> GSFVGSIDQGTTSSRFLIFNGEGNPVASHQIEFENLYPKSGWHEQDPYELLNSVQQCIDGAMHKFASLGYSKENIRAIGITNQRETTVVWDSVTGEPLHNAIVWPDTRTSALVRELKARQSADSLLELCGLPLSTYPSSVKLLWLIQNVDAVKQAYEEGRLAFGTVDSWLIYKLNGGAQAERPIHVTDSTNASRTMFMNLRTLQYDDKLLGFFGIDRNKIKLPKIVPSSDPEAFGKVATGALAGVPIAGCLGDQSSALVGQCGFSPGQAKNTYGTGCFLLYNVGTEPVISKYGLLATVAYDFGRGRKPVYALEGSIAVAGAGITFLMNNLGFAPKPSEINALAESVLDNGGVVFVTAFSGLFAPYWIDDAKGTLFGITQHTTKGHIARATLEATCYQTRAILDAMEKDSGHKLESLAVDGGLSASDLCMQTQADISGIPVDRPRMRETTALGAAIAAGLATGVWRELDHVKESIAGGANGNGKKNAREVFYPKMDRKKAERLFRKWEQAVEMSRGWVREQEEEDGE

Here, we report the first structure of glycerol kinase from the thermophilic filamentous fungus Chaetomium thermophilum (CtGK). Glycerol kinase (EC 2.7.1.30) catalyzes the transfer of phosphate moiety from ATP to glycerol to form glycerol 3-phosphate (G3P). Overall, the CtGK polypeptide chain can be divided into two distinct domains classified by Pfam as FGGY_N (residues 65–325) and FGGY_C (residues 331–583) connected by a flexible region. A similar case is found in CtGK, which forms extended dimers via the interaction between the C-terminal domains with a prominent contribution from hydrophobic residues (Phe422, Gly436, Phe389, Leu394, Thr437, Phe439, Gly440, Ile441, Thr437, Thr445, Leu438, Ile450, Trp580).

Subsequently, by replacing the cryoprotectant solution with 20–25% glycerol, we were able to solve the enzyme-substrate complex with a clear electron density that could be attributed to the bound glycerol moiety. In total, three different crystal structures were obtained in the presence of glycerol, constituting 13 polypeptide chains. Generally, the same extent of the chain could be modeled as in the apo structures, i.e., for residues 65–583 with an approximate 9aa gap between H18 and B18. The substrate is bound in an evolutionarily conserved cleft within the N-terminal domain that opens towards the C-terminal domain. The glycerol molecule is coordinated by polar interactions with side chains of Glu149, Arg 148, Asp317, Gln318, and additionally with Arg148 main-chain amide. The carbon chain of glycerol packs against hydrophobic Trp168 and Phe342. A similar mode of binding was described previously for P. falciparum GK, where Phe271 and Tyr135 undergo shift upon substrate or cofactor binding. However, the movement of equivalent residues (Phe342 and Tyr200) was not observed in either of the presented CtGK complexes. Of note, we solved and refined five CtGK structures, and each of them belongs to a different space group, despite crystals having grown in the same buffer condition. We observed that in the absence of nucleotide, CtGK adopts open conformation, which upon nucleotide binding closes up.>SRRSRSEILQDVLSRCSPLNIPIEDDQPVKVSFEYSLQKIFRADVENDEVDIGLWTTLVWKDRCLNWFNEFTSFKELTVPIAEIWTPDIFIFDSVGAPEIFSDKLARVSQDGTVTYVPQLKVRLSCPLADLKLETGVTCSLKSGSWTHSTQELTLE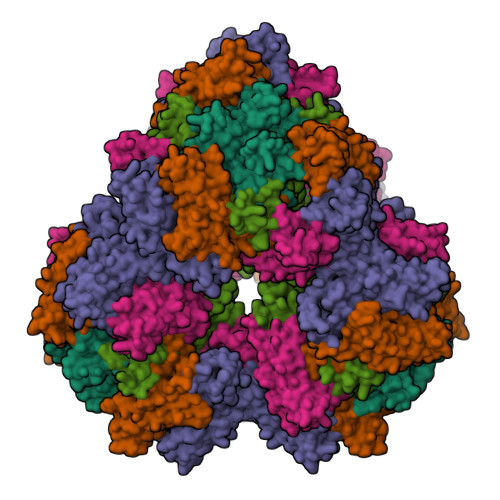VNAKVDLGDYASDTRFQLLNATQQVNRKQYPCCPETYEDTTLSFTFRKP[5x]>[2x]CCGGG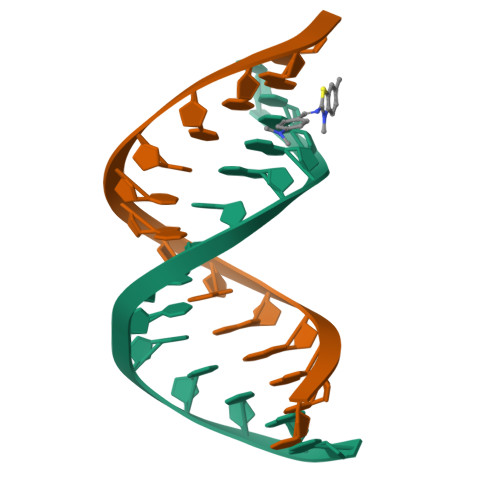GTACCCCGG> GAADKGEIRVGNRYQADITDLLKEGEEDGRD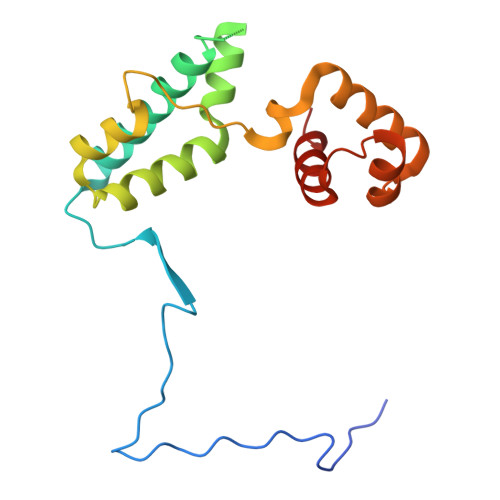QSRLETQVWEAHNPLTDKQIDQFLVVARSVGTFARALDCSSSVRQPSLHMSAAAASRDITLFHAMDTLHKNIYDISKAISALVPQGGPVLCRDEMEEWSASEANLFEEALEKYGKDFTDIQQDFLPWKSLTSIIEYYYMWKTTDR2-[5-bromanyl-3-cyano-6-methyl-4-(trifluoromethyl)pyridin-2-yl]oxy-~{N}-ethyl-~{N}-(3-methylphenyl)ethanamide 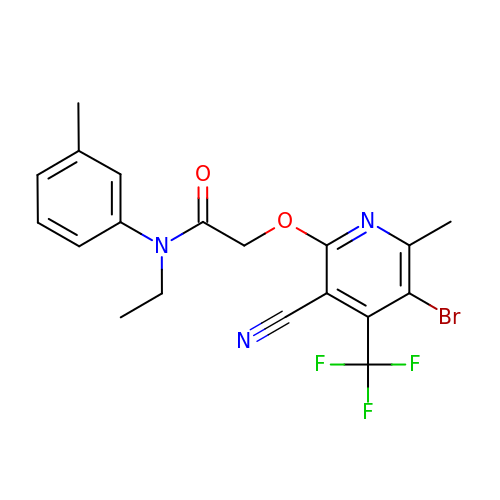| C19 H17 Br F3 N3 O2 | OFTSRQPYUSQTEG-UHFFFAOYSA-N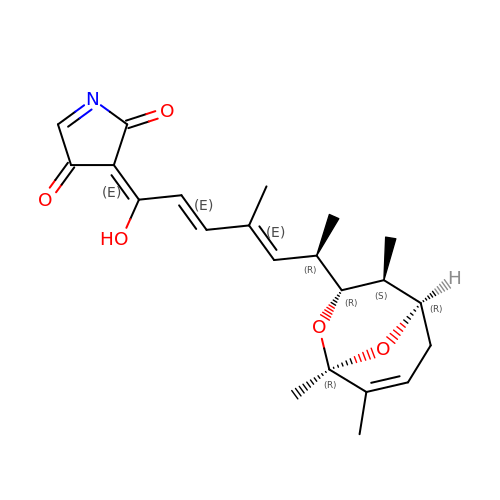(3E)-3-{(2E,4E,6R)-1-hydroxy-4-methyl-6-[(1R,3R,4S,5R)-1,4,8-trimethyl-2,9-dioxabicyclo[3.3.1]non-7-en-3-yl]hepta-2,4-dien-1-ylidene}-2H-pyrrole-2,4(3H)-dione | C22 H27 N O5 | MHIKRZGCDBIVFG-IVGQTCGHSA-N> ACGGA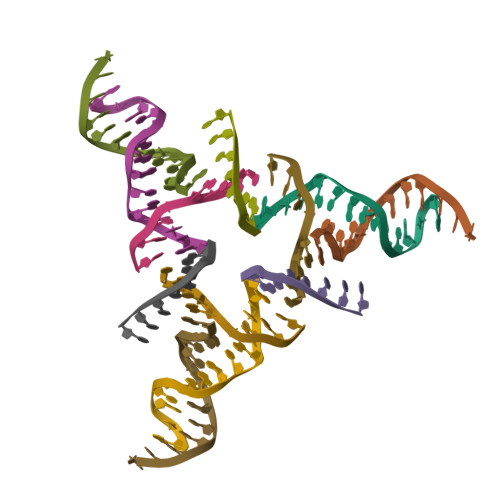CAGAGTGCA;> CACACCGT;> GGTGCACTCTGTG;> CCCTGTG>[2x]SELNEKLATAWEGFTKGDWQNEVNVRDFIQKNYTPYEGDESFLAGATEATTTLWDKVMEGVKLENRTHAPVDFDTAVASTITSHDAGYINKQLEKIVGLQTEAPLKRALIPFGGIKMIEGSCKAYNRELDPMIKKIFTEYRKTHNQGVFDVYTPDILRCRKSGVLTGLPDAYGRGRIIGDYRRVALYGIDYLMKDKLAQFTSLQADLENGVNLEQTIRLREEIAEQHRALGQMKEMAAKYGYDISGPATNAQEAIQWTYFGYLAAVKSQNGAAMSFGRTSTFLDVYIERDLKAGKITEQEAQEMVDHLVMKLRMVRFLRTPEYDELFSGDPIWATESIGGMGLDGRTLVTKNSFRFLNTLYTMGPSPEPNMTILWSEKLPLNFKKFAAKVSIDTSSLQYENDDLMRPDFNNDDYAIA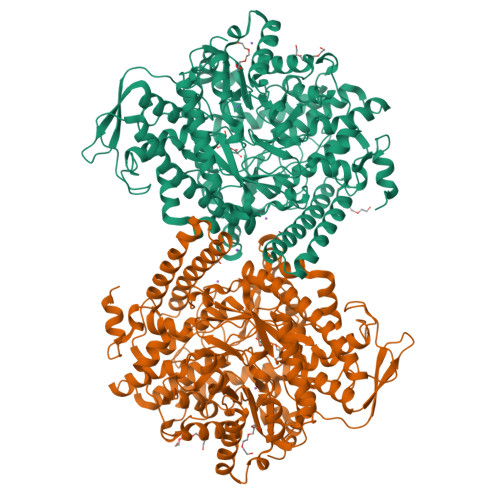CCVSPMIVGKQMQFFGARANLAKTMLYAINGGVDEKLKMQVGPKSEPIKGDVLNYDEVMERMDHFMDWLAKQYITALNIIHYMHDKYSYEASLMALHDRDVIRTMACGIAGLSVAADSLSAIKYAKVKPIRDEDGLAIDFEIEGEYPQFGNNDPRVDDLAVDLVERFMKKIQKLHTYRDAIPTQSVLTITSNVVYGKKTGNTPDGRRAGAPFGPGANPMHGRDQKGAVASLTSVAKLPFAYAKDGISYTFSIVPNALGKDDEVRKTNLAGLMDGYFHHEASIEGGQHLNVNVMNREMLLDAMENPEKYPQLTIRVSGYAVRFNSLTKEQQQDVITRTFTQSM> VTS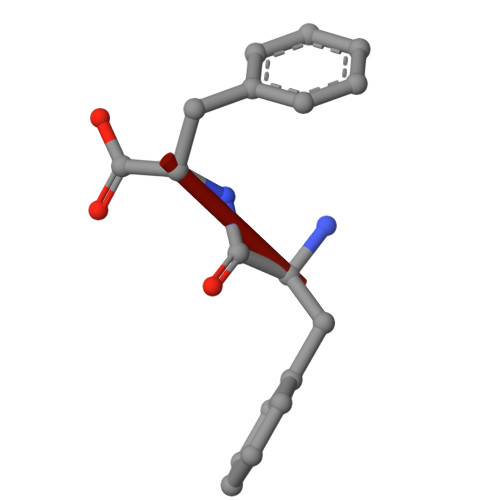FF(2R)-2-aminohexanedioic acid | C6 H11 N O4 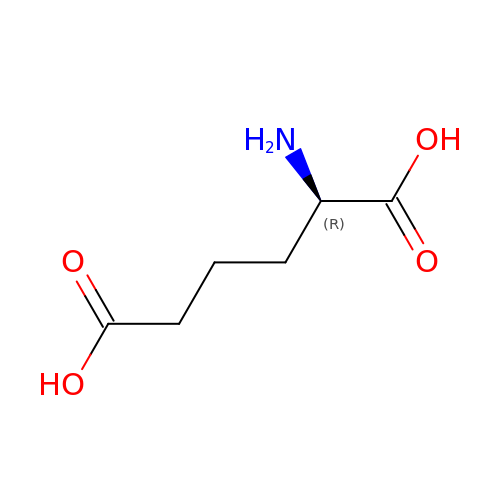| OYIFNHCXNCRBQI-SCSAIBSYSA-N>[3x]MTRPDNEPARLRSVAENLAAEAAAFVRGRRAE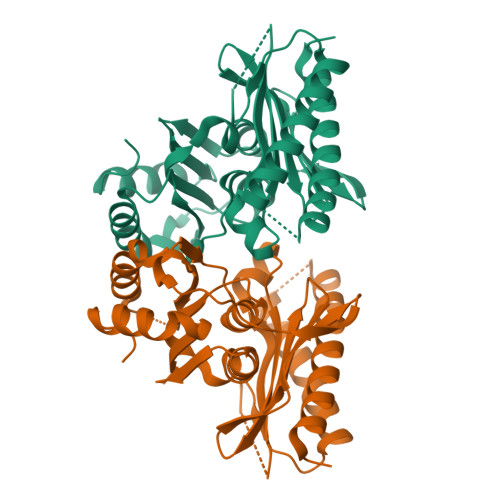VFGISRAGDGDGAVRAKSSPTDPVTVVDTDTERLLRDRLAQLRPGDPILGEEGGGPADVTATPSDRVTWVLDPIDGTVNFVYGIPAYAVSIGAQVGGITVAGAVADVAARTVYSAATGLGAHLTDERGRHVLRCTGVDELSMALLGTGFGYSVRCREKQAELLAHVVPLVRDVRRIGSAALDLCMVAAGRLDAYYEHGVQVWDCAAGALIAAEAGARVLLSTPRAGGAGLVVVAAAPGIADELLAALQRFNGLEPIPDALEHHHHHH>TIAALLS[2x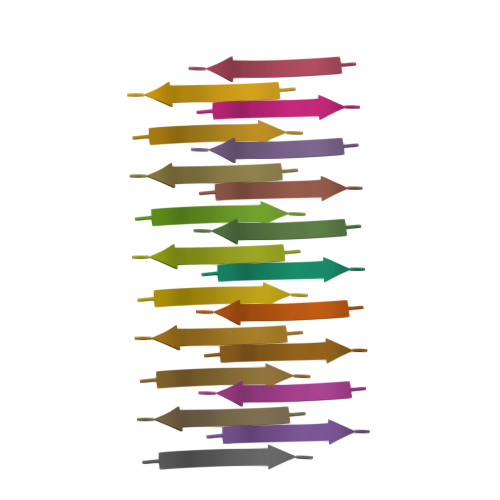]> GLKPEMIEKLNEQMNLELYSSLLYQQMSAWCSYHGFEGAAAFLRRHAQEEMTHMQRLFDYLTDTGNLPRIDTIPSPFAEYSSLDELFQETYKHEQLITQKINELAHAAMTNQDYPTFNFLQWYVAEQHEE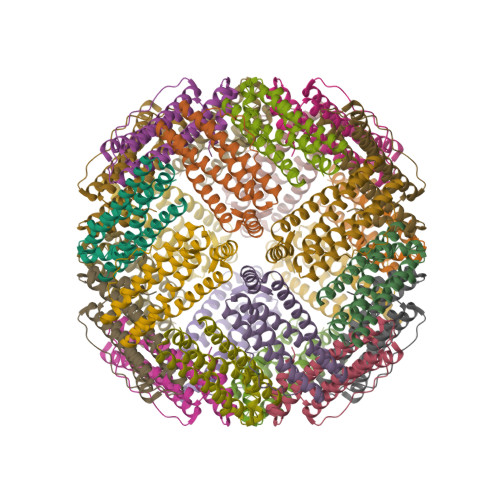EKLFKSIIDKLSLAGKSGEGLYFIDKELSTLDT8-AMINO-3-QUINOLINOL | C9 H8 N2 O | 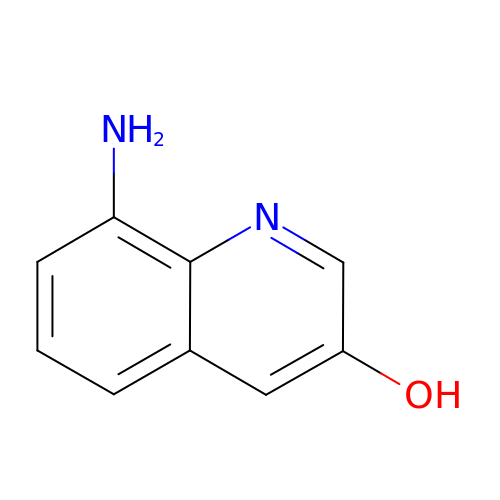GLVURCUKRZAGQN-UHFFFAOYSA-N N-{4-[4-(2-amino-4-oxo-3,4-dihydro-5H-pyrrolo[3,2-d]pyrimidin-5-yl)butyl]-2-fluorobenzoyl}-L-glutamic 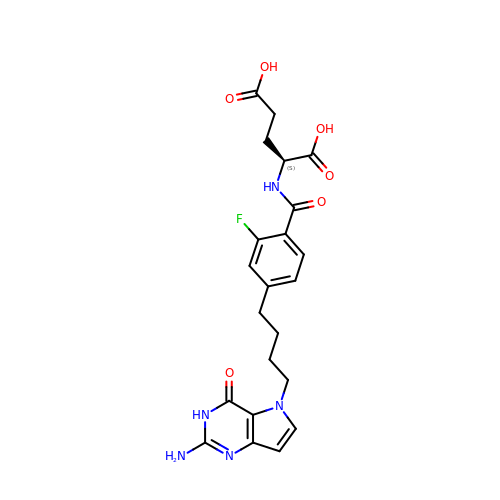acid | C22 H24 F N5 O6 | XKLSPKTUYQAZHW-INIZCTEOSA-N The GTPase Rab1 is a master regulator of the early secretory pathway and is critical for autophagy. Rab1 activation is controlled by its guanine nucleotide exchange factor, the multisubunit TRAPPIII complex. While the TRAPPII and TRAPPIII complexes share a core set of subunits, the distinguishing feature of the TRAPPIII complex is the presence of the Trs85 subunit (TRAPPC8 in metazoans) (Sacher et al, 1998, 2000, 2001, 2019; Lynch‐Day et al, 2010). Our results show that the Trs85 subunit serves as a membrane anchor, via its amphipathic helix, for the entire TRAPPIII complex.

Here, we report the high‐resolution structure of the intact yeast TRAPPIII complex bound to its substrate GTPase Rab1/Ypt1, representing the key intermediate of the nucleotide exchange reaction. Although these data were of lower quality due to the higher tilt angle, combination of data from the three tilt angles provided sufficient orientation coverage to generate a 3.7 Å reconstruction suitable for de novo model building from 69,315 particles (EV2C–G and EV3). The TRAPPIII complex adopts a narrow rod‐like structure, in agreement with the published negative‐stain EM structure. The cryo‐EM structure reveals that the N‐terminal portion of Trs85 adopts a GTPase‐like fold and the C‐terminal portion folds into a twisting α‐solenoid comprising five pairs of α‐helices. The GTPase‐like fold in Trs85 has multiple insertions relative to a typical GTPase protein and does not appear capable of binding nucleotide. There are two interfaces between Trs85 and the TRAPP core subunits: an extensive interaction between Trs85 and Trs20, involving 31 residues and encompassing a total surface area of roughly 2,250 Å, and a much smaller interaction between Trs31 and part of a largely unstructured loop of Trs85. The interface between Trs85 and Trs20 is quite conserved and involves Trs20 Asp46, a residue known to be important for assembly of both the TRAPPII and TRAPPIII complexes that is mutated in spondyloepiphyseal dysplasia tarda (SEDT). Some small differences were noted; for example, we observed covalently bound palmitate molecules in both Bet3 subunits, whereas only one of the Bet3 subunits appeared to be bound to palmitate in the previous structure of the catalytic core. In our cryo‐EM reconstruction of the TRAPPIII‐GTPase complex, we observed a region of strong but unexpected density on the surface of the complex that we have confidently assigned as corresponding to a portion of the Rab1/Ypt1 HVD (and EV4H).

> MNSEYDYLFKLLLIGNSGVGKSCLLLRFSDDTYTNDYISTIGVDFKIKTVELDGKTVKLQIWDTAGQERFRTITSSYYRGSHGIIIVYDVTDQESFNGVKMWLQEIDRYATSTVLKLLVGNKCDLKDKRVVEYDVAKEFADANKMPFLETSALDSTNVEDAFLTMARQIKESMSQQNLNETTQKKEDKGNVNLKGQSLTNTGGGCC;> MGSSHHHHHHSQENLYFQGMVFSYEHYMNLLFHLDNSKETVPPEIAKRIISNAIAPVITVTSTPLFDKHIQETYKVDSLYMLLRFFGGCVSDRDQANEAKVGQHEHEVCDASDSTDSIPKNKNLEVPNLSKKGSRSRSNSLFQRDSTQSQYIRFTRPLGDLIETRDANDMLFNYHSLEVFLDNYLKLVAANTDEMVPHNLLKKSIYHSFFSLAISSTNNLSPYETFNHPILSLIALDISNGEVYEDARDLLVNFKNLNHNTENFPIFMNTNEMLPVFLLCYNDDSQEEFEKCQALAKKLKKQLFVESILLALWKDSFIYDENSVIQLHQPVMSSLEEILFFLQAPTQTTLSLALINSIYDMLDYLVYDLMIPFMKRKVSFWEETILQPRKSLFNGAKFFKKFMNKNPVNGNHQHNSLTRDSQGNEYFASSSSEFLMRKLADWSMMLSDFKTAYSTYESLMDDLDAFPKYLASCIEWCAVSLLMGAQSIVTVKMIKNDINPLIERALATYENCSRIQRGKGKESNSLDVTEPVRSYETRCMILASELFLSLSNTWTSTPYAIQYLETILDECKLGPCSQIMVWERLSDCYNLRVDPRIKHRVGAMKKDAKDTEDLRGEHKYSTDHFTDEDILSEGLTRRRKAAFFRLIAAKKWAEQKQWRQVSWCLKDIESTYSEIKFLHGNGLILSKLKNQLNLKDVDSAPRPSEKNLTRTSVSFIG;> MSSTHSNNVGHPQSSPQGPLTEQQRAQQQYQIFENSLPKVSQSVYQMLLNEMVPLAMGIERQISGDVISSDSNVTSENGNINNMIKRLKIEEHHTVDIIRSHNLIHELYKADEEEKEKVLARLRNIGFQIGLKLSELLIFSNNPNLKFKEMDLLLIMKFICRDVWKQIFGKQIDNLKTNHRGTFYLLDYDYRPIQSFSLEEDAKNEELKMIEPFLEIPVGIIRGVLSSLGYSSEEVICLASFIDRPTDRPKTAFPKGVSFHVQVTMPQ;>MVSTTQSRSLKAMGEEIWKNKTEKINTELFTLTYGSIVAQLCQDYERDFNKVNDHLYSMGYNIGCRLIEDFLARTALPRCENLVKTSEVLSKCAFKIFLNITPNITNWSHNKDTFSLILDENPLADFVELPMDAMKSLWYSNILCGVLKGSLEMVQLDCDVWFVSDILRGDSQTEIKVKLNRILKDEIPIGED[2x];> MGIYSFWIFDRHCNCIFDREWTLASNSASGTINSKQNEEDAKLLYGMIFSLRSITQKLSKGSVKNDIRSISTGKYRVHTYCTASGLWFVLLSDFKQQSYTQVLQYIYSHIYVKYVSNNLLSPYDFAENENEMRGQGTRKITNRNFISVLESFLAPMVNQ;> MAIETILVINKSGGLIYQRNFTNDEQKLNSNEYLILASTLHGVFAIASQLTPKALQLTQQTNIENTIPYIPYVGMSSNRSDTRNGGGNNNKHTNNEKLGSFKGDDFFKEPFTNWNKSGLRQLCTDQFTMFIYQTLTGLKFVAISSSVMPQRQPTIATTDKPDRPKSTSNLAIQIADNFLRKVYCLYSDYVMKDPSYSMEMPIRSNLFDEKVKKMVENLQ;> MSQRIIQPSASDQQFPGKSDGYEYTVGPKQAITSEASTTYIPSRIYSESLLFKRQEASLSAMAFLFQEMISQLHRTCKTAGDFETKLSDYGHNIGIRLLELLNFRASVSPSSLPRASAFLSQNESSSKLSNASNSPGMLANSSTATSASANERLQEKQTESLSNYITKMRRRDLKILDILQFIHGTLWSYLFNHVSDDLVKSSERDNEYMIVDNFPTLTQFIPGENVSCEYFVCGIIKGFLFNAGFPCGVTAHRMPQGGHSQRTVYLIQFDRQVLDREGLRFG;> MPQYFAIIGKKDNPVYEIEFTNAENPQGFPQDLKELNPFILHASLDIVEDLQWQINPTSQLNGNGGNGSNGGGGFLRSRAVNNTDNCYLGKVDHFYGLAITAYISYSGMKFVMIHGNSANSSVVIDDNNMRSFYQEVHELYVKTLMNPFYKITDPIRSPAFDSRVRTLARKHLSK>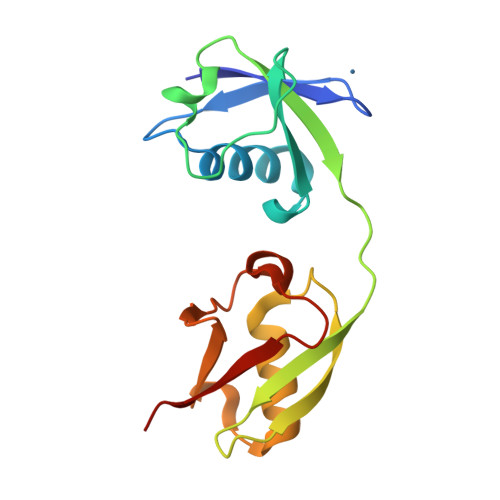 MGWDLTVKMLAGNEFQVSLSSSMSVSELKAQITQKIGVHAFQQRLAVHPSGVALQDRVPLASQGLGPGSTVLLVVDKSDEPLSILVRNNKGRSSTYEVRLTQTVAHLKQQVSGLEGVQDDLFWLTFEGKPLEDQLPLGEYGLKPLSTVFMNLRLR> DKRTQIVYSDDVYKENLV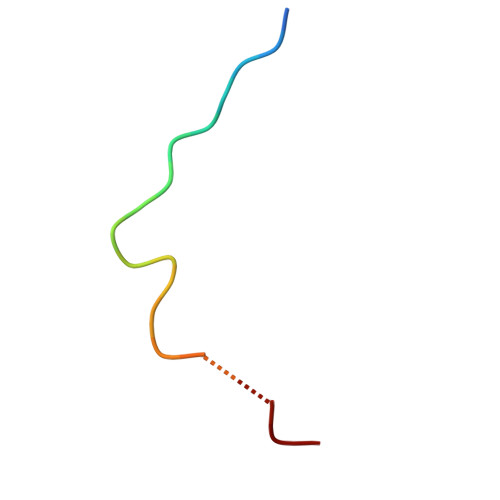DGF> HKILHR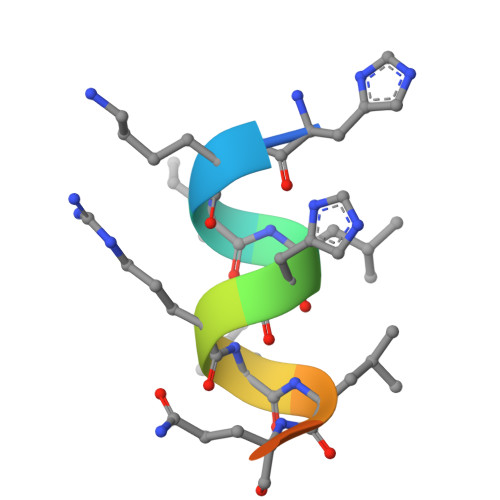LLQEGS> AFSYSSAAGGESKKILGVFFAAHEYAKNPEFLGCVENALGIREWLESKGHKYVVTSDKDGPDSELD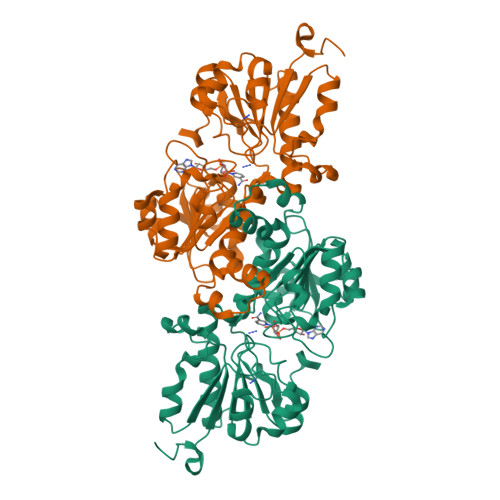KELADAHILITTPFHPAYMTKERLAKAKNLELLVTAGVGSDHIDLHAAAEKGLTVSEVTGSNVTSVAEDEVLRILVLVRNFAPGWKQVSEGGWNVAAVVHHAYDLIDRTVGTVGGGRIGQELMKRLKGFGLKEMLYYDRNSLGAEREKELGCKRETDLDTMLSKCDVVVVNTPLTDQTRGLFNKERIAKMKKGAYLVNNARGAIADTEAVKEACESGHLGGYGGDVWNAQPAGKDHPWRYMPNHAMTPHISGTTLDAQKRFAAGTKDMIDRWLKHEAFPEQNYIVREGKLASQYL> GSPVRQGARPAGAAIVPGQIAAARLTPVAWQQVPGWQDDSLIGATIALRQNCARLARQANWQRACAAAMRLDDLDVGSARTFFETYFTPFQFANNDGTLDGLVTGYYEPLLHGSRVRRGPYQYALYRWPAG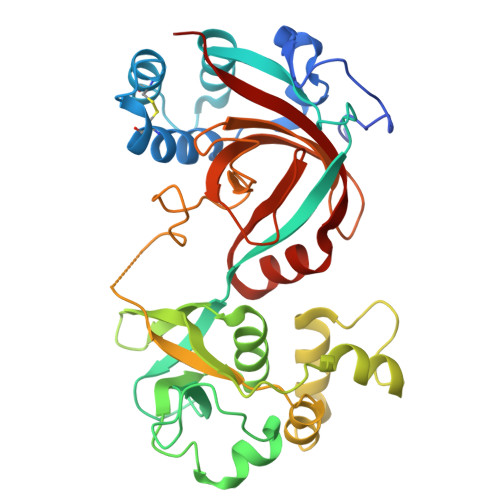YRAGASMPARAQLMRSGALSGNELVWVDDPIEAFFLQVQGSGRVVLDDGTVMRVGYGGTNNQPYRSIGKWLLDHGELGAGQATMQGIKAWARANPSRVDALLDTNPRFVFFREMPSQEDVPHGGADGPVGALGVPLTPERSIAVDPSSIPLGTPVFLQTTRPMTNAPLNRLVFAQDVGTAIKGGVRADYFWGLGDDAGDQAGRMKQNGRMWLLFPNS>[2x]GTSSMADIGSISDNYSSLLQVSEALGRAGLESSNLIVGIDFTKSNEWTGAKSFNRKSLHHLSNTPNPYEQAITIIGRTLAAFDEDNLIPCYGFGDASTHDQDVFSFYPEGRFCNGFEEVLARYREIVPQLKLAGPT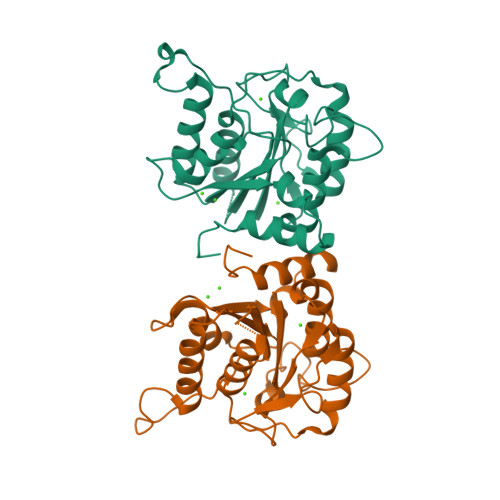SFAPIIEMAMTVVEQSSGQYHVLVIIADGQVTRSVDTEHGRLSPQEQKTVDAIVKASTLPLSIVLVGVGDGPWDMMQEFDDNIPARAFDNFQFVNFTEIMSKNKDQSRKETEFALSALMEIPPQY(R)-2-(3-([1,1'-Biphenyl]-4-carbonyl)-3-(4-methylbenzyl)ureido)-3-((cyclohexylmethyl)sulfonyl)propanoic acid | C32 H36 N2 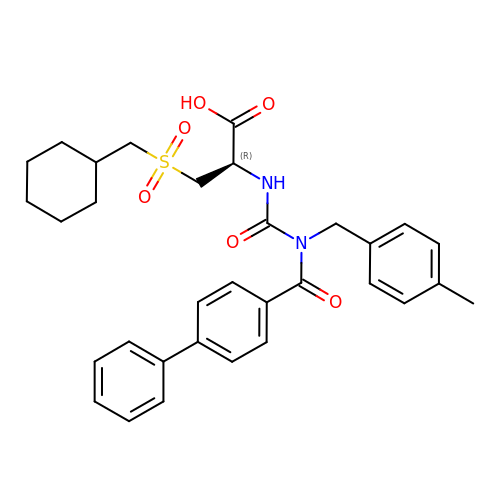O6 S | TZBNSZNCLWFKOH-LJAQVGFWSA-N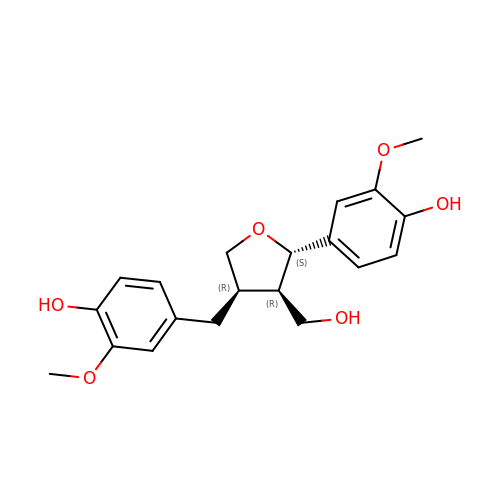4-[[(3R,4R,5S)-4-(hydroxymethyl)-5-(3-methoxy-4-oxidanyl-phenyl)oxolan-3-yl]methyl]-2-methoxy-phenol | C20 H24 O6 | MHXCIKYXNYCMHY-AUSJPIAWSA-N> QEERNQQQDDIEELETKAVGMSNDGRFLKFDIEIGRGSFKTVYKGLDTETTVEVAWCELQERKLTKSERQRFKEEAEMLKGLQHPNIVRFYDSWESTVKGKKCIVLVTELMTSGTLKTYLKRFKVMKIKVLRSWCRQILKGLQFLHTRTPPIIHRDLKCDNIFIT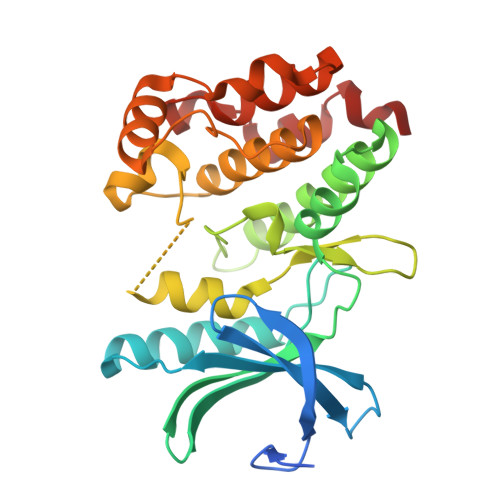GPTGSVKIGDLGLATLKRASFAKSVIGTPEFMAPEMYEEKYDESVDVYAFGMCMLEMATSEYPYSECQNAAQIYRRVTSGVKPASFDKVAIPEVKEIIEGCIRQNKDERYSIKDLLNHAFFQEET>[2x]MSESPMFAANGMPKVNQGAEEDVRILGYDPLASPALLQVQIPATPTSLETAKRGRREAIDIITGKDDRVLVIVGPCSIHDLEAAQEYALRLKKLSDELKGDLSIIMRAYLEKPRTTVGWKGLINDPDVNNTFNINKGLQSARQLFVNLTNIGLPIGSEMLDTISPQ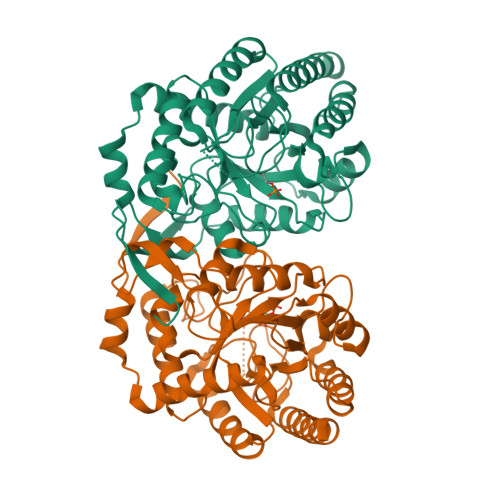YLADLVSFGAIGARTTESQLHRELASGLSFPVGFKNGTDGTLNVAVDACQAAAHSHHFMGVTKHGVAAITTTKGNEHCFVILRGGKKGTNYDAKSVAEAKAQLPAGSNGLMIDYSHGNSNKDFRNQPKVNDVVCEQIANGENAITGVMIESNINEGNQGIPAEGKAGLKYGVSITDACIGWETTEDVLRKLAAAVRQRREVNKK>[2x]MTNR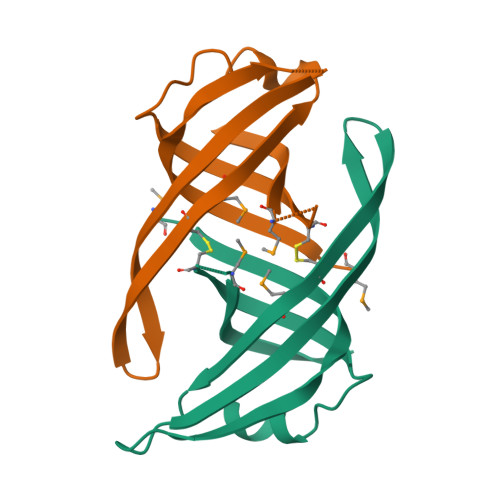LVLSGTVCRAPLRKVSPSGIPHCQFVLEHRSVQEEAGFHRQAWCQMPVIVSGHENQAITHSITVGSRITVQGFISCHKAKNGLSKMVLHAEQIELIDSGD> MINGSKRIAQPIRWAMVGGGRNSQIGYIHRSAALRDQSFALVAGAFDIDPGRGREFGVQLGVDPQRCYPDYRTLFEQEARRPDGIQAVSVATPNGTHFAITRAALEAGLHVVCEKPLCFTLEEAETLREIALANNRVVGVTYGYAGHQLIEQARAMIADGELGEIRMVHMQFAHGFHSAPVEGQNEATKWRVDPRLAGPSYVLGDVGTHPLYLSEVMLPEFRIKRLMCSRQSFVKSRAPLEDNAYTLMEYEGGAMGLVWSSAVNAGSMHGQKIRVIGSRASLEWWDEHP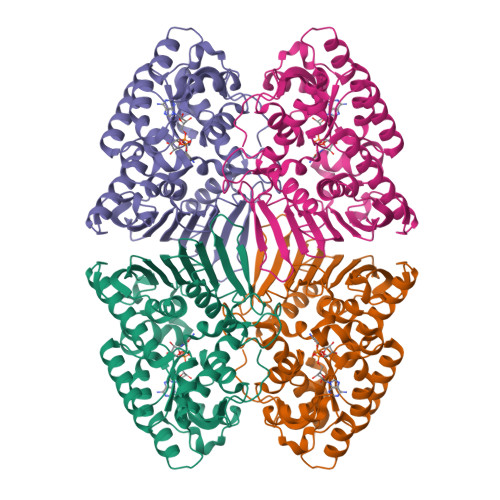NQLAFEIQGQPVQVLERGMGYLHPGALLDDRIGAGHPEGLFEAWSNLYYRFAMAMDATERGDGALLAGLRYPDIHAGVEGVRWVERCVQSADRGGVWVDYLEHHHHHH>MTYPLLTRKTLMKKTPLALLLTLGLLQTPLAAFAATAPLDLVGPVSDYKIYVTENIEELVSHTQKFTDAVKKGDIATAKKLYAPTRVYYESVE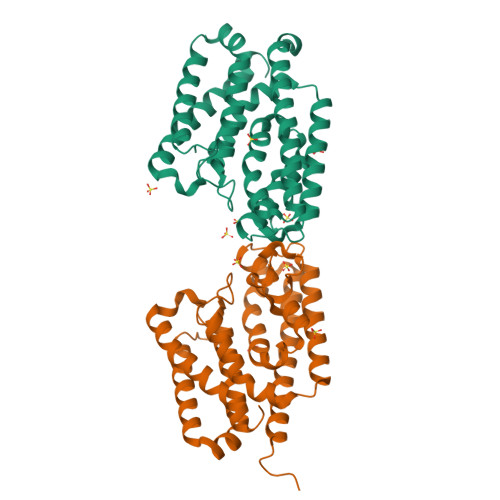PIAELFSDLDASIDSRVDDHEQGVAAEDFTGFHRLEYALFSQNTTKDQGPIADKLLSDVKDLEKRVADLTFPPEKVVGGAAALLEEVAATKISGEEDRYSHTDLYDFQGNIDGAKKIVDLFRPQIEQQDKAFSSKVDKNFATVDKILAKYKTKDGGFETYDKVKENDRKALVGPVNTLAEDLSTLRGKLGLN[2x]> GAMSSPAGSPT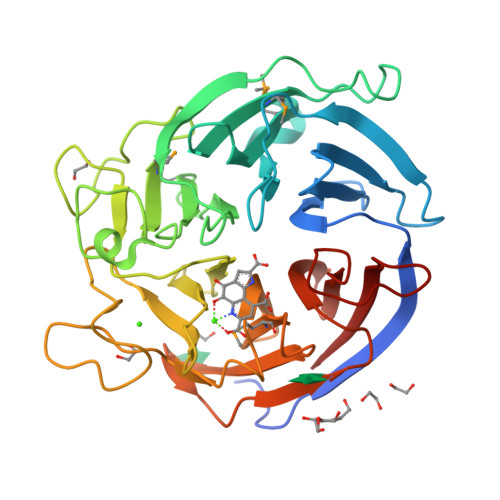EQAPPAKGSVKVLRTVATGLNSPWGLAPLPGGDLLVSSRDEATITRVDAKTGRKTELGEVPGVSPSGEGGLLGIALSPDYASDHMVYAYFTSASDNRIVRMLYDEKKPSGEQLGAPDTVFRGIPKGVIHNGGRIAFGPDKMLYAGTGESGDTGLSQDRKSLGGKILRMTPDGEPAPGNPFPGSPVYSYGHRNVQGLAWDDKQRLFASEFGQDTWDELNAIKPGDNYGWPEAEGKGGGSGFHDPVAQWSTDEASPSGIAYAEGSVWMAGLRGERLWRIPLKGTAAAADPQAFLEGEYGRLRTVAPAGGDKLWLVTSNTDGRGDAKGGDDRILELEVE> MIVVDIAIVLVAIAAVLSSYRMIRGPHAGDRAIAADLLFFAFIALLALVGVRVDS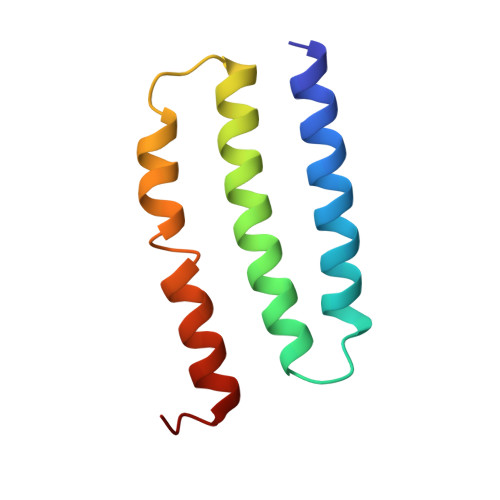PFVYDLVLVATLVGLVSALSLARLMSGGRR>GSHMEEKLAVSLQEALQEGDTRALREVLEEIHPQDLLALWDELKGEHRYVVLTLLPKAKAAE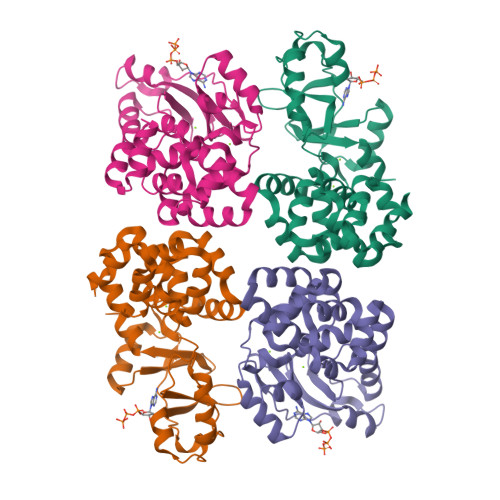VLSHLSPEEQAEYLKTLPPWRLREILEELSLDDLADALQAVRKEDPAYFQRLKDLLDPRTRAEVEALARYEEDEAGGLMTPEYVAVREGMTVEEVLRFLRRAAPDAETIYYIYVVDEKGRLKGVLSLRDLIVADPRTRVAEIMNPKVVYVRTDTDQEEVARLMADYDFTVLPVVDEEGRLVGIVTVDDVLDVLEAEATEDIHKLGAVDVPDLVYSE[4x]> MFTGLVEAIGVVKDVQGTIDNGFAMKIEAPQILDDCHTGDSIAVNGTCLTVTDFDRYHFTVGIAPESLRLTNLGQCKAGDPVNLERAVLSSTRMGGHFVQGHVDTVAEIVEKKQDGEAIDFTFRPRDPFVLKYIVYKGYIALDGTSLTIT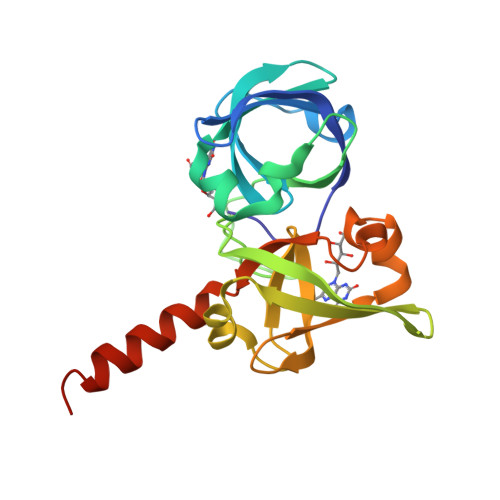HVDDSTFSIMMISYTQSKVIMAKKNVGDLVNVEVDQIGKYTEKLVEAHIADWIKKTQA> MAVAVGMIETLGFPAVVEAADAMVKAARVTLVGYEKIGTGRVTVIVRGDVSEVQASVSAGTESVKRVNGGQVLSTHIIARPHENLEYVLPIRYTEE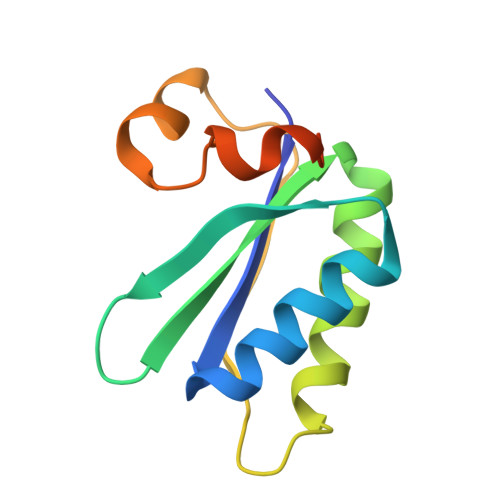VEQFREGVGTPRNITRQ>GSHMKDGKPGPLVDDKGRFFKPLQGDSRGEIEVKFYESFSSNTEVPEHIHRYFPVYHGTQAVEGSDGAAMMVLENLLAEYTKPSVMDVKMGSRTWYPDASEEYIQKCLKKDTGTTTVSSGFRISGFEVYDHKESSFWKPERKLLRGLDVDGARLTLRKFVSSNSLSDTGSKPDSAFASSVYGGSHGILTQLLELKTWFENQTLYHFNSCSILMVYENESILKGNDDDARPQVKLVDFAHVLDGNGVIDHNFLGGLCSFINFIR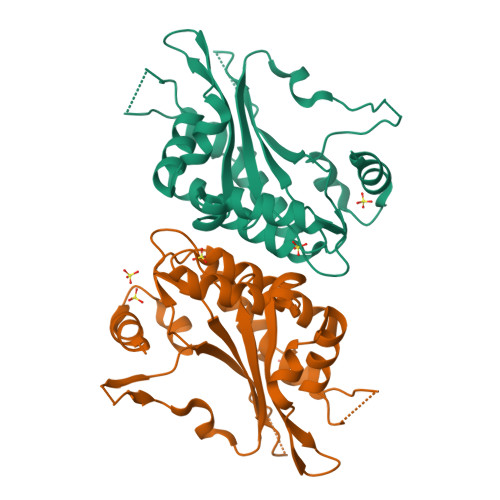EILQSPDESADS[2x]SETD3 is a selective actin histidine methyltransferase that catalyses mono-methylation of actin at histidine 73 (actin H73me) to regulate actin function. SETD3 belongs to a subclass of protein methyltransferases that in addition to containing the catalytic SET domain, also have a Rubisco-substrate binding (RSB) domain that is present in the plant enzyme RLSMT (Rubisco large subunit methyltransferase). We have previously identified the actin histidine methyltransferase SETD3 as a critical host factor physically interacting with the viral protease 2A. Through unbiased genetic screens, we have previously identified SETD3 as critically important for the replication of a broad range of enteroviruses, including genetically diverse rhinoviruses, coxsackieviruses, poliovirus, and the non-polio enteroviruses EV-D68 and EV-A71, which are associated with severe neuropathogenesis.

We determined the SETD3-CV-B3 2A complex structure to 3.5 Å resolution by cryo-electron microscopy (cryo-EM) and observed clear density for residues 22-495 of SETD3 and 4-141 of 2A protease. CV-B3 2A binds in the pocket formed by the SET domain and the RSB domain of SETD3, forming two separate interaction interfaces with SETD3. The interaction surface areas with the SET domain and the RSB domain, including the linker, are 747 Å2 and 460 Å2, respectively. The linker region connecting the SET domain and the RSB domain contributes two hydrogen bonds/salt bridge contacts between SETD3 R336 and 2A E74. In contrast, the interaction surface with the SET domain is much larger and includes a small hydrophobic core area centred on interactions between SETD3 residues Q257 and P259, and 2A residue V59. Additionally, a pair of main-chain main-chain hydrogen bonds between SETD3 Y288 and 2A H68 form part of an anti-parallel intermolecular β-sheet structure between the two proteins. Although we do not observe any overlap of actin and 2A binding in the SETD3 active site, actin peptide residues 66-72 and 2A partially overlap in the substrate binding region, forming intermolecular β-sheets with SETD3 involving SETD3 residue Y288. Compared to the high-affinity binding between WT SETD3 and 2A (KD = 47 nM), a single mutation of Y288P in the SET domain (SET288) reduces binding affinity 53-fold (KD = 2.5 µM) and a double mutation in the same domain, SET257+266, 213-fold (KD = 10 µM). In addition, the presence of an actin substrate peptide inhibits the binding of SETD3 to 2A in vitro. Mutations in the RSB domain interface have only minor effects on 2A binding and no effect on viral replication, while mutations of key contact residues in the SET interface show severely reduced binding affinity to 2A and completely abrogate viral replication.

> SNAGKKSRVKTQKSGTGATATVSPKEILNLTSELLQKCSSPAPGPGKEWEEYVQIRTLVEKIRKKQKGLSVTFDGKREDYFPDLMKWASENGASVEGFEMVNFKEEGFGLRATRDIKAEELFLWVPRKLLMTVESAKNSVLGPLYSQDRILQAMGNIALAFHLLCERASPNSFWQPYIQTLPSEYDTPLYFEEDEVRYLQSTQAIHDVFSQYKNTARQYAYFYKVIQTHPHANKLPLKDSFTYEDYRWAVSSVMTRQNQIPTEDGSRVTLALIPLWDMCNHTNGLITTGYNLEDDRCECVALQDFRAGEQIYIFYGTRSNAEFVIHSGFFFDNNSHDRVKIKLGVSKSDRLYAMKAEVLARAGIPTSSVFALHFTEPPISAQLLAFLRVFCMTEEELKEHLLGDSAIDRIFTLGNSEFPVSWDNEVKLWTFLEDRASLLLKTYKTTIEEDKSVLKNHDLSVRAKMAIKLRLGEKEILEKAVKSAAVNREYYRQQMEEKAPLPKYEESNLGLLESSVGDSRLPLVLRNLEEEAGVQDALNIREAISKAKATENGLVNGENSIPNGTRSENESLNQESKRAVEDAKGSSSDSTAGVKE;> SNAMGQQSGAVYVGNYRVVNRHLATSADWQNCVWESYNRDLLVSTTTAHGCDIIARCQCTTGVYFCASKNKHYPISFEGPGLVEVQESEYYPRRYQSHVLLAAGFSEPGDAGGILRCEHGVIGIVTMGGEGVVGFADIRDLLWLEDDAMEQ> MHHHHHHSSRENLYFQGANSLSVHQLAAQGEMLYLATRIEQENVINHTDEEGFTPLMWAAAHGQIAVVEFLLQNGADPQLLGKGRESALSLACSKGYTDIVKMLLDCGVDVNEYDWNGGTPLLYAVHGNHVKCVKMLLESGADPTIE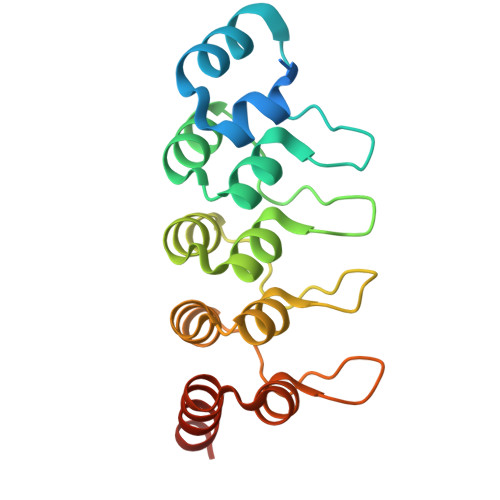TDSGYNSMDLAVALGYRSVQQVIESHLLKLLQNIKE>[2x]MGSSHHHHHHSSGLVPRGSHMPSASASRKSQEKPREIMDAAEDYAKERYGI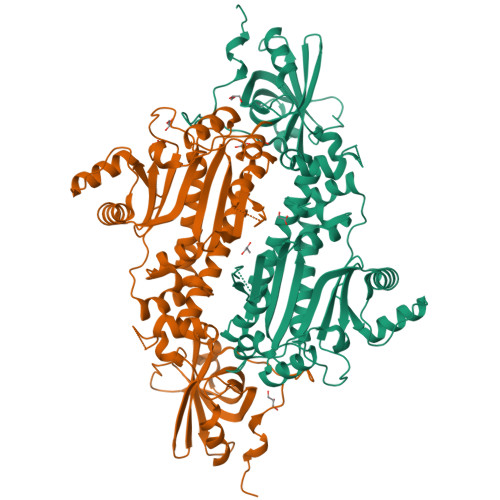SSMIQSQEKPDRVLVRVRDLTIQKADEVVWVRARVHTSRAKGKQCFLVLRQQQFNVQALVAVGDHASKQMVKFAANINKESIVDVEGVVRKVNQKIGSCTQQDVELHVQKIYVISLAEPRLPLQLDDAVRPEAEGEEEGRATVNQDTRLDNRVIDLRTSTSQAVFRLQSGICHLFRETLINKGFVEIQTPKIISAASEGGANVFTVSYFKNNAYLAQSPQLYKQMCICADFEKVFSIGPVFRAEDSNTHRHLTEFVGLDIEMAFNYHYHEVMEEIADTMVQIFKGLQERFQTEIQTVNKQFPCEPFKFLEPTLRLEYCEALAMLREAGVEMGDEDDLSTPNEKLLGHLVKEKYDTDFYILDKYPLAVRPFYTMPDPRNPKQSNSYDMFMRGEEILSGAQRIHDPQLLTERALHHGIDLEKIKAYIDSFRFGAPPHAGGGIGLERVTMLFLGLHNVRQTSMFPRDPKRLTP> VPAFLGKLWALVGDPGTDHLIRWSPSGTSFLVSDQSRFAKEVLPQYFKHSNMASFVRQLNMYGFRKVVSIEQGGLLRPE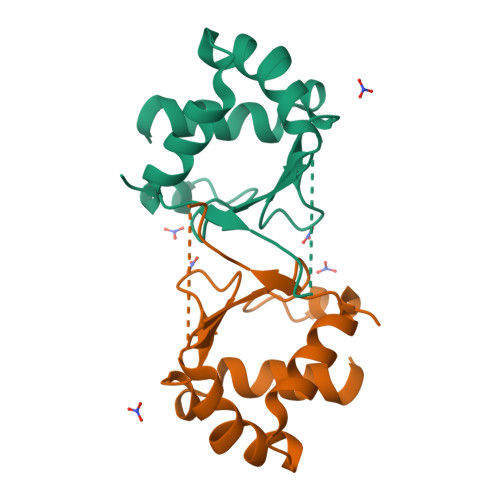RDHVEFQHPSFVRGREQLLERVRRKV> NPVERYVDEVLNEVLVVPNINQSHPTTSNAAPVLDAAETGHTNKIQPEDTIETRYVQSSQTLDEMSVESFLGRSGCIHESVLDIVDNYNDQSFTKWNINLQEMAQIRRKFEMFTYARFDSEITMVPSVAAKDGHIGHIVMQYMYVPPGAPIPTTRDDYAWQSGTNASVFWQHGQPFPRFSLPFLSIASAYYMFYDGYDGDTYKSRYGTVVTNDMGTLCSRIVTSEQLHKVKVVTRIYHKAKHTKAWCPRPPRAVQYSHTHTTNYKLSSEVHNDVAIRPRTNLTTV;> SPSVEACGYSDRIIQITRGDSTITSQDVANAVVGYGVWPHYLTPQDATAIDKPTQPDTSSNRFYTLDSKMWNSTSKGWWW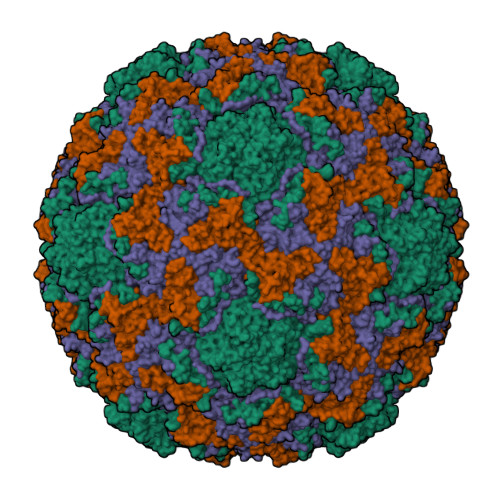KLPDALKDMGIFGENMFYHFLGRSGYTVHVQCNASKFHQGTLLVVMIPEHQLATVNKGNVNAGYKYTHPGEAGREVGTQVENEKQPSDDNWLNFDGTLLGNLLIFPHQFINLRSNNSATLIVPYVNAVPMDSMVRHNNWSLVIIPVCQLQSNNISNIVPITVSISPMCAEFSGARAKTVVQ;> GLPVYVTPGSGQFMTTDDMQSPCALPWYHPTKEIFIPGEVKNLIEMCQVDTLIPINSTQSNIGNVSMYTVTLSPQTKLAEEIFAIKVDIASHPLATTLIGEIASYFTHWTGSLRFSFMFCGTANTTLKVLLAYTPPGIGKPRSRKEAMLGTHVVWDVGLQSTVSLVVPWISASQYRFTTPDTYSSAGYITCWYQTNFVVPPNTPNTAEMLCFVSGCKDFCLRMARDTDLHKQTGPITQ;> GAQVSRQNVGTHSTQNMVSNGSSINYFNINYFKDAASSGASRLDFSQDPSKFTDPVKDVLEKGIPTLQ>[4x]GEIQWMRPSKEVGYPIINAPSKTKLEPSAFHYVFEGVKEPAVLTKNDPRLKTDFEEAIFSKYVGNKITEVDEYMKEAVDHYAGQLMSLDINTEQMCLEDAMYGTDGLEALDLSTSAGYPYVAMGKKKRDILNKQTRDTKEMQKLLDTYGINLPLVTYV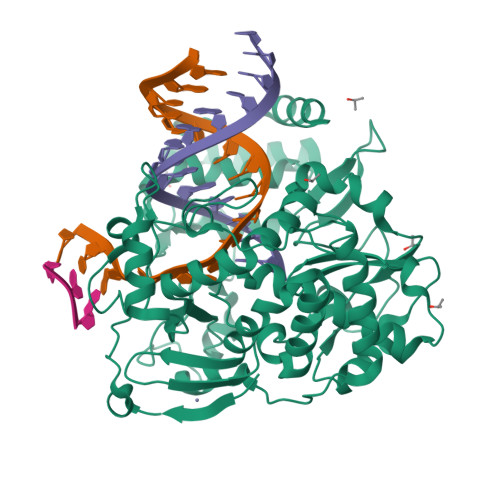KDELRSKTKVEQGKSRLIEASSLNDSVAMRMAFGNLYAAFHKNPGVITGSAVGCDPDLFWSKIPVLMEEKLFAFDYTGYDASLSPAWFEALKMVLEKIGFGDRVDYIDYLNHSHHLYKNKTYCVKGGMPSGCSGTSIFNSMINNLIIRTLLLKTYKGIDLDHLKMIAYGDDVIASYPHEVDASLLAQSGKDYGLTMTPADKSATFETVTWENVTFLKRFFRADEKYPFLIHPVMPMKEIHESIRWTKDPRNTQDHVRSLCLLAWHNGEEEYNKFLAKIRSVPIGRALDLPEYSTLYRRWLDSFGSSSHHHHHH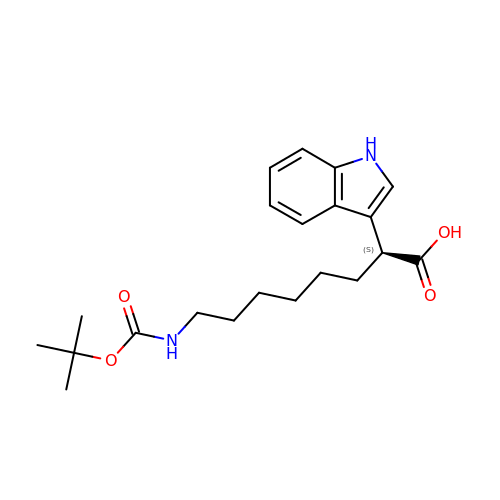(2S)-8-[(tert-butoxycarbonyl)amino]-2-(1H-indol-3-yl)octanoic acid | C21 H30 N2 O4 | AWVCKFLATUTBCX-INIZCTEOSA-N>GSTAAEKPKLHYFNARGRMESTRWLLAAAGVEFEEKFIKSAEDLDKLRNDGYLMFQQVPMVEIDGMKLVQTRAILNYIASKYNLYGKDIKERALI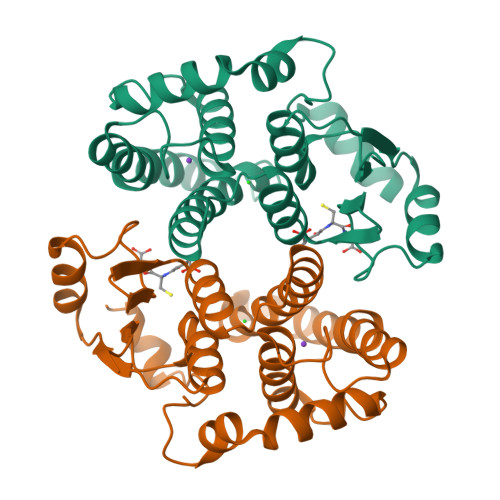DMYIEGIADLGEMILLLPVCPPEEKDAKLALIKEKIKNRYFPAFEKVLKSHGQDYLVGNKLSRADIHLVELLYYVEELDSSLISSFPLLKALKTRISNLPTVKKFLQPGSPRKPPMDEKSLEEHRKIFRF[2x]> DLTVSLIPVSGLKAGKNAPSAKIAKLVVNSTTLKEFGVRGISNNVVDS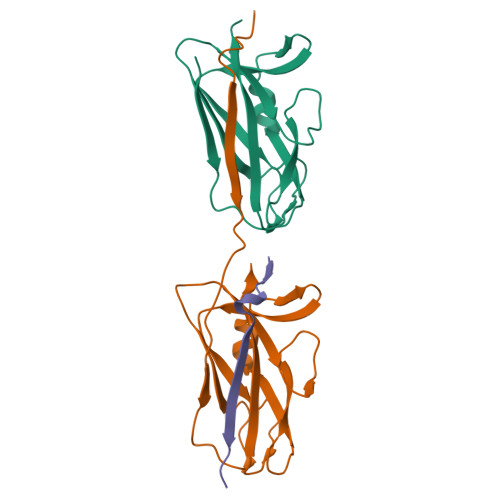TGTAWRVAGKNTGKEIGVGLSSDSLRRSDSTEKWNGVNWMTFNSNDTLDIVLTGPAQNVTADTYPITLDVVGYQP;> GSFLPNSEQQKSVDIVFSSPQDLTVSLIPVSGLKAGKNAPSAKIAKLVVNSTTLKEFGVRGISNNVVDSTGTAWRVAGKNTGKEIGVGLSSDSLRRSDSTEKWNGVNWMTFNSNDTLDIVLTGPAQNVTADTYPITLDVVGYQP;> GSFLPNSEQQKSVDIVFSS>[2x]GSHMAKMSAENEIEMRICDYLRRHGRSTVQD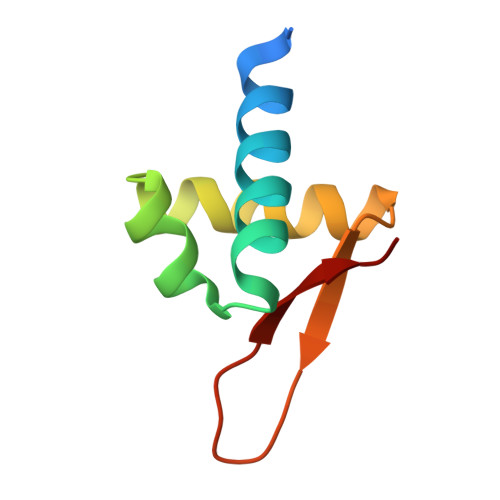IFKELKLEKSTVNRHLYSLQASKQVFKTVEDNKRPVWDLVE>MQWSGARALEALLTVAGELRGPPLQLDTGQLLKIAKRGGVTAVEAVHAWRNALTGAPLNLTPEQVVAIASHDGGKQALETVQRLLPVLCQAHGLTPQQVVAIASHDGGKQALETVQRLLPVLCQAHGLTPEQVVAIASHDGGKQALETVQALLPVLCQAHGLTPEQVVAIASNGGGKQALETVQRLLPVLCQAHGLTPQQVVAIASNGGGKQALETVQRLLPVLCQAHGLTPQQVVAIASNGGGKQALETVQRLLPVLCQAHGLTPQQVVAIASNRGGKQALETVQRLLPVLCQAHGLTPQQVVAIASNGGGKQALETVQRLLPVLCQAHGLTPQQVVAIASHDGGKQALETVQRLLPVLCQAHGLTPEQVVAIASNGGGKQALETVQRLLPVLCQAHGLTPEQVVAIASHDGGKQALETVQRLLPVLCQAHGLTPQQVVAIASNGGGRPALESIVAQLSRPDPALAALTNDHLVALACLGGRPALDAVKKLEHHHHHH[2x]

Transcription activator-like (TAL) effectors specifically bind to double stranded (ds) DNA through a central domain of tandem repeats. Each TAL effector (TALE) repeat comprises 33–35 amino acids and recognizes one specific DNA base through a highly variable residue at a fixed position in the repeat. The crystal structures of TAL effector (TALE) proteins bound to their respective target DNAs have revealed that the residue at position 13 is the only one directly involved in DNA base recognition, whereas the 12th residue stabilizes the proper loop conformation. dHax3, an engineered TALE protein, proved to be a useful scaffold for structural characterizations. We then present fifteen crystal structures of engineered dHax3 variants in complex with target DNA molecules, which elucidate the structural basis for the recognition of bases adenine (A) and guanine (G) by reported or uncharacterized TALE codes.

When the natural TALE codes were discovered, no code was found highly specific for base G. In light of the structures of the DNA-binding zinc finger proteins where positive charged amino acids such as Arg, His, Lys play a critical role in the coordination of base G, we made a dHax3 variant with an Arg34, His34, Lys34 in the 7th repeat. We then attempted to co-crystallize these proteins with a modified dHax3 box element whose 7th base is changed from A to G. Four complex structures were determined at high resolutions.> GMEGPLNLAH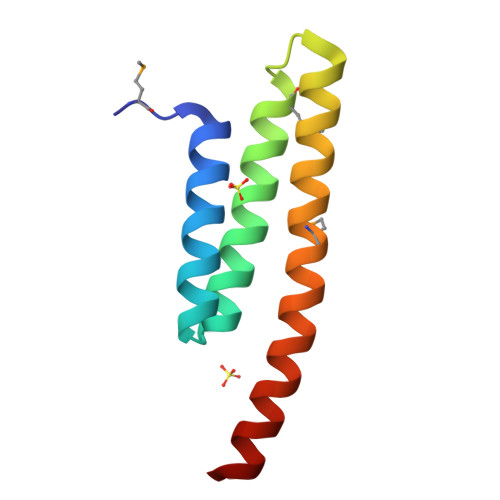QQSRRADRLLAAGKYEEAISCHKKAAAYLSEAMKLTQSEQAHLSLELQRDSHMKQLLLIQERWKRAQREERLKA>ASMTGGQQMGRGSSLTACPEESPLLVGPMLIEFNIPVDLKLVEQQNPKVKLGGRYTPMDCISPHKVAIIIPFRNRQEHLKYWLYYL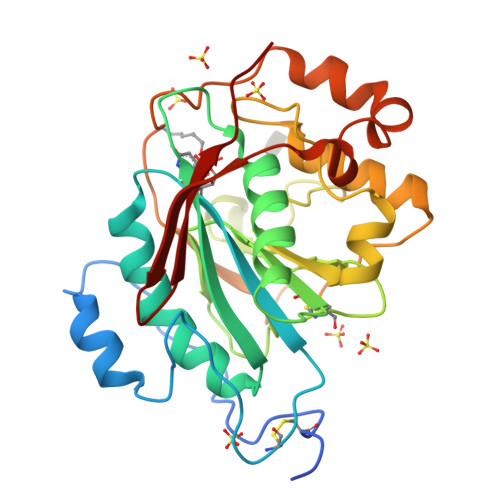HPILQRQQLDYGIYVINQAGESMFNRAKLLNVGFKEALKDYDYNCFVFSDVDLIPMNDHNTYRCFSQPRHISVAMDKFGFSLPYVQYFGGVSALSKQQFLSINGFPNNYWGWGGEDDDIYNRLAFRGMSVSRPNAVIGKTRHIRHSRDKKNEPNPQRFDRIAHTKETMLSDGLNSLTYMVLEVQRYPLYTKITVDIGTPS[2x]> MRAEDLPKAVVFLEPQWYRVLEKDSVTLKCQGAYSPEDQSTRWFHNESLISSQTSSYFIAAARVNNSGEYRCQTSLSTLSDPVQLEVHIGWLLLQAPRWVFKEEESIHLRCHSWKNTLLHKVTYLQNGKGRKYFHQNSDFYIPKATLKDSGSYFCRGLIGSKNVSSETVQITITQDLAVSSISSFFPPGYQV

In these mechanisms, the effectiveness of inactivation depends upon Fc gamma receptors (FcγRs) expressed at the surface of effector cells and the interaction of the extracellular domain of the FcγR with the Fc portion of the antibody bound to its cognate epitope. In contrast to humans, macaques only have one low affinity FcγRIII receptor, CD16, which shares a polymorphism at position 158 with human FcγRIIIa with Ile158 and Val158 variants. Similar to human low affinity FcγR receptors, the macaque FcγRIII receptor consists of two immunoglobulin-like domains packed against one another at a roughly 80-90 degree angle in a comma- or apostrophe-like shape. The Mm FcγRIII forms an asymmetric complex with macaque IgG1 Fc with the Fc binding near the bend in the comma-shaped receptor; the majority of the receptor’s contact residues to the Fc reside on the C-terminal second immunoglobulin-like (d2) domain closer to the cell membrane.

We also determined the high-resolution structure of the Mm FcγRIII(Ile158) variant alone (apo), not complexed with Fc. In structural studies, we used receptor variants in which glycosylation sites at Asn38 and Asn169 (two of the five total) were removed by mutagenesis to aid in crystallization. The apo macaque FcγRIII(Ile158) receptor, expressed as Val158 variant, was crystallized in orthorhombic space group P212121 with cell dimensions a = 49.1 Å, b = 67.0 Å, and c = 69.7 Å. Crystals diffracted to 1.9 Å resolution with one receptor in the asymmetric unit. The model was refined to an R/Rfree of 0.182/0.218. While one well-ordered glycan can be seen attached to Asn45 in the apo macaque receptor structure, no glycan is visible linked to Asn162 due to disorder. In addition, there is a hydrogen bond between the Asn45 linked glycan mannose on domain 1 and Glu166 on domain 2 which is only visible in the apo receptor structure due to its higher resolution and better resolved glycan density. This added hydrogen bond may provide an explanation for the detrimental effect of removing this glycan on expression. Receptor crystals were grown from 25% PEG 3350 and 0.1 M HEPES pH 7.0.> KKKK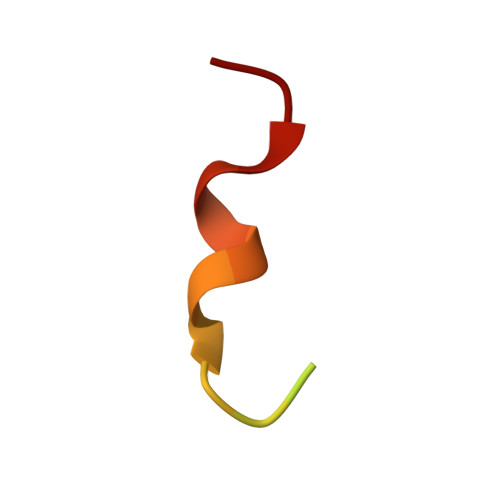KKEEEVDLSGLSGMFGF A nuclease belonging to the GIY-YIG superfamily has been identified from A. thaliana (At-HIGLE: HYL-1 Interacting GIY-YIG Like Endonuclease) (AT2G30350). At-HIGLE comprises an N-terminal GIY-YIG nuclease domain (amino acid residues 1–183) and an extended C-terminal region (amino acid residues 184-368). Here, we elucidated the crystal structure of the At-HIGLE nuclease domain from Arabidopsis thaliana, establishing it as a member of the SLX1-lineage of the GIY-YIG superfamily with structural changes in DNA interacting regions. Unlike fungal SLX1, At-HIGLE exists as a catalytically active homodimer capable of generating two coordinated nicks during HJ resolution.

Eventually, At-HIGLE was truncated (At-HIGLE1–183) based on secondary structure predictions to remove disordered segments at the C-terminal end. At-HIGLE1–183 crystallized in P212121 space group with one molecule in the asymmetric unit. Crystals diffracted to a resolution of 1.7 Å. The structure exhibits a mixed α/β topology. At-HIGLE1–183 comprises of a β sheet formed by five β strands oriented as β2–β1–β3–β4–β5 with β2 and β3 strands present in anti-parallel orientations with respect to β1, β4 and β5 strands. Poor electron densities did not allow the modeling of amino acids 1–26 at the N-terminal end and 180–183 at the C-terminal end. At-HIGLE1–183 superimposes with the nuclease domain of Cg-SLX1 with a root-mean square deviation (r.m.s.d.) of 0.8 Å. Compared to the nuclease domain of Cg-Slx1, At-HIGLE1–183 showed differences in the conformation of loops relevant to DNA substrate binding. In summary, At-HIGLE exists in a conformation ready for interactions with DNA substrate. Catalytically essential amino acid residues are Glu95, Arg55, Tyr31 and Tyr45.

> MREKRGNRKALDPVGEDGVTGKDGKGFFACYLLTSLSPRHKGQTYIGFTVNPRRRIRQHNGEITSGAWRTKKKRPWEMVLCIYGFPTNVSALQFEWAWQHPRESVAVREAAAAFKSFSGVASKIKLVYTMLNLPAWNSLNLTVNYFSSKYAHHGGKSPSLPLHMKVQVCAMEDLQYFTKVDDS>LPVEKIIR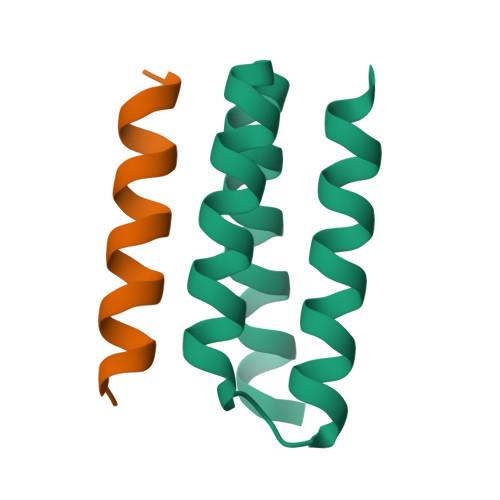EAKKILDELLKRGLIDPELARIAREVLERARKLGNEEAARFVLELIERLRRELS[2x];>DEHELLETAARWFYEIAKRA[2x]>[12x]MHHHHHHDPPCEELEIVWKNIKAEARALADCEPMLASFYHATLLKHENLGSALSYMLANKLASPIMPAIAIREVVEEAYAADPEMIASAACDIQAVRTRDPAVDKYSTPLLYLKGFHALQAYRIGHWLWNKGRRALAIFLQNQVSVSFQVDIHPAAKIGRGIMLDHATGIVVGETAVIEDDVSILQSVTLGGTGKTSGDRHPKIREGVMIGAGA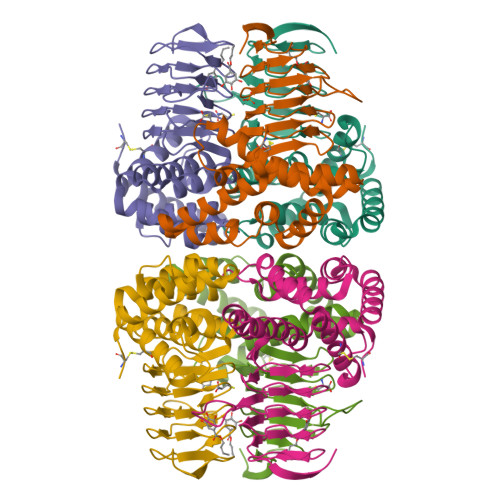KILGNIEVGRGAKIGAGSVVLQPVPPHTTAAGVPARIVGKPGSDKPSMDMDQHFNGIHHTFEYGDG> MKQKVHSVSYLAKAEFEYKNGVYDL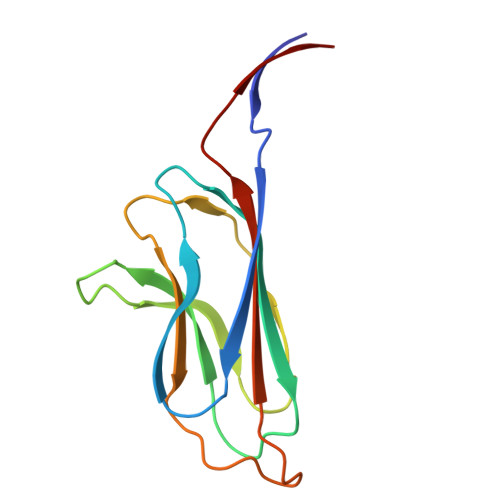VALPTGAEVIKISLEVVGLPTAGHVSVGFKDESKKNYSSILTLPVNETSGVVTKDYTVKSDKIVAAEVKDALAEGSDGRPVKCVLRALYFLPSVIEVEY> MAHHHHHHMIKTPDEIEKMRIAGRLAAEVLDMIKPHIKAGVSTLELDTICRNHIENVQHAIPACVGYGGAPGRPAFQHSICTSVNHVVCHGIPSENKILKNGDILNIDVTVIKDGYHGDTNMMYIVGGETSILANRLCKVAQEAMYRGMATVRDGSYLGDIG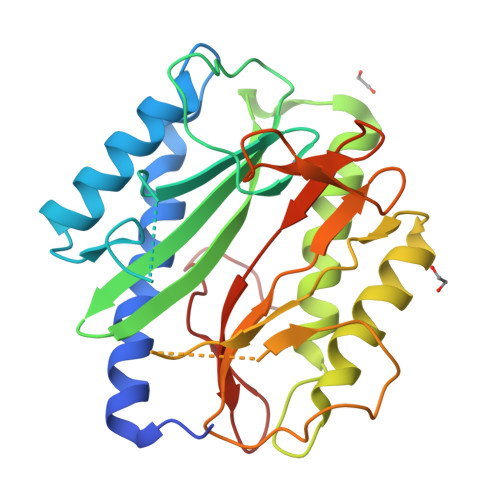HAIQKYVESERFSVVREYCGHGIGTVFHDEPQVLHYGQAGTGMRLEAGMTFTIEPMVNAGVWQTKLLGDKWTVVTKDHKLSAQYEHTILVTKTGIEVLTARPEEDLSR>[3x]MPKFDVSKSDLER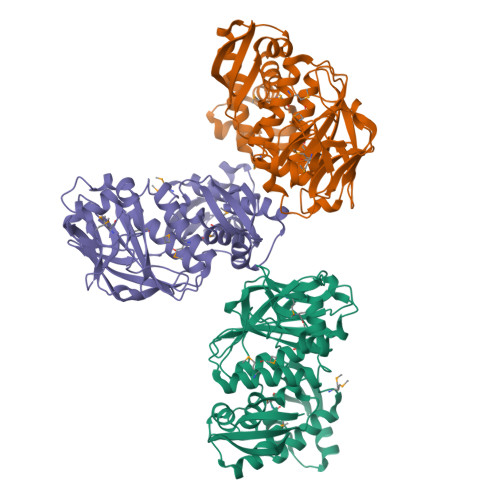LIGRSFSIEEWEDLVLYAKCELDDVWEENGKVYFKLDSKDTNRPDLWSAEGVARQIKWALGIEKGLPKYEVKKSNVTVYVDEKLKDIRPYGVYAIVEGLRLDEDSLSQMIQLQEKIALTFGRRRREVAIGIFDFDKIKPPIYYKAAEKTEKFAPLGYKEEMTLEEILEKHEKGREYGHLIKDKQFYPLLIDSEGNVLSMPPIINSEFTGRVTTDTKNVFIDVTGWKLEKVMLALNVMVTALAERGGKIRSVRVVYKDFEIETPDLTPKEFEVELDYIRKLSGLELNDGEIKELLEKMMYEVEISRGRAKLKYPAFRDDIMHARDILEDVLIAYGY>SMSANENNLIWIDLEMTGLDPERDRIIEIATLVTDANLNILAEGPTIAVHQSDEQLALMDDWNVRTHTASGLVERVKASTMGDREAELATLEFLKQWVPAGKSPICGNSIGQDRRFLFKYMPELEAYFHYRYLDVSTLKE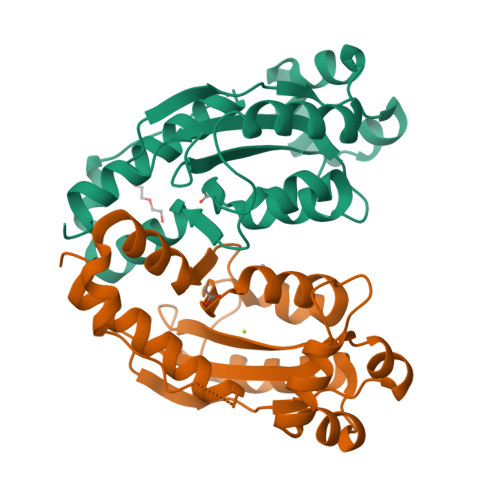LARRWKPEILDGFTKQGTHQAMDDIRESVAELAYYREHFIKL[4x]>[2x]KGNEFEDYCLKRELLMGIFEMGWEKP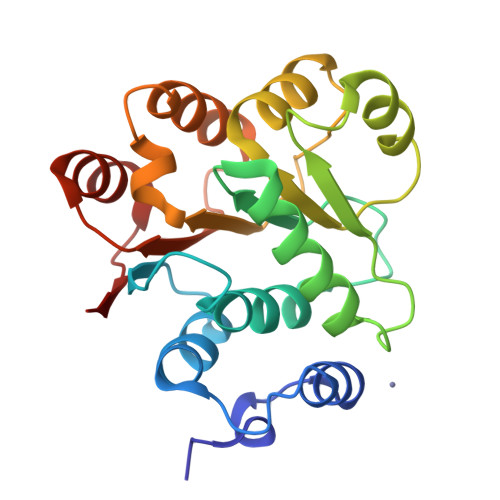SPIQEESIPIALSGRDILARAKNGTGKSGAYLIPLLERLDLKKDNIQAMVIVPTRELALQVSQICIQVSKHMGGAKVMATTGGTNLRDDIMRLDDTVHVVIATPGRILDLIKKGVAKVDHVQMIVLDEADKLLSQDFVQIMEDIILTLPKNRQILLYSATFPLSVQKFMNSHLEKPYEIN>[4x]MGSMSDLQQHALNYYRQQQLPSGWADLFGVIVNGMMDNAGEREGLA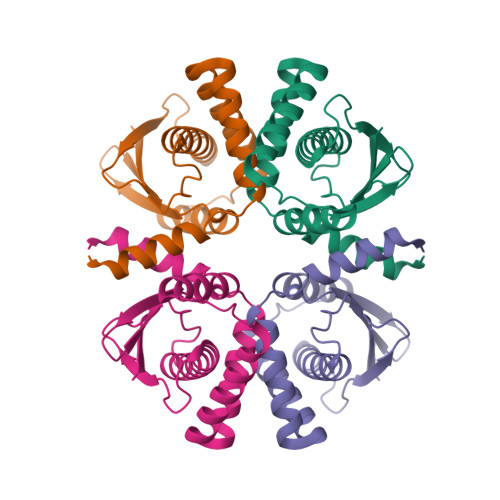FLRHIGGQLAERYPLPAAVTVVDLEREINRVLSLFHWGCVDLRPYENRLEIYHLALPASVNSSGSVRWRMAMAAVLQGLYSRWLREQGGVESVPLSCEETDSESTLLFRYQH> LEIWELKKDVYVVELDWYPDAPGEMVVLTCDTPEEDGITWTLDQSSEVLGSGKTLTIQVKEFGDAGQYTCHKGGEVLSHSLLLLHKKEDGIWSTDILKDQKEPKNKTFLRCEAKNYSGRFTCWWLTTISTD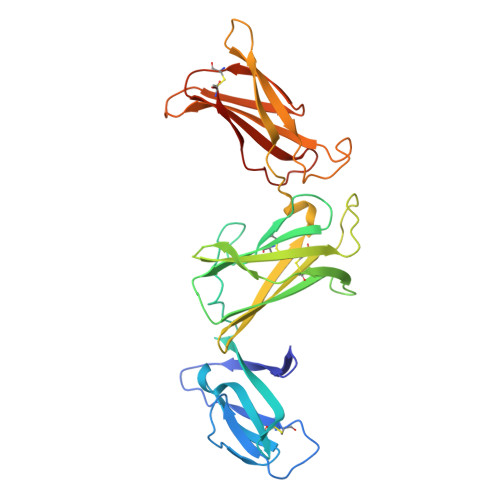LTFSVKSSRGSSDPQGVTCGAATLSAERVRGDNKEYEYSVECQEDSACPAAEESLPIEVMVDAVHKLKYENYTSSFFIRDIIKPDPPKNLQLKPLKNSRQVEVSWEYPDTWSTPHSYFSLTFCVQVQGKSKREKKDRVFTDKTSATVICRKNASISVRAQDRYYSSSWSEWASVPCSHHHHHH[(1S)-1-{[6-(3-chloro-4-methylphenyl)thieno[2,3-d]pyrimidin-4-yl]amino}-2-phenylethyl]phosphonic acid | C21 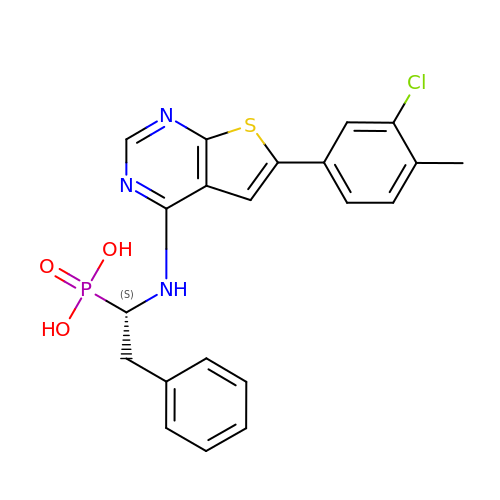H19 Cl N3 O3 P S | FHHLLOYGUMAOOP-IBGZPJMESA-N>VNVLGGIEYSINNATLCSVGFSVTRGATKGFVTAGHCGGVGAIVRIGGTQVGSFAARVFPGNDRAWVSVGSAHTLQGAVSNYSGGTIAIRGSAEAAIGAAVCRSGRTTGYRCGNITAKNVTANYAEGAVRGLTQGNACMGRGDSGGSWFTSAGQAQGVMSGGNVQSNGNNCGIPASQRSSLFERVGPILSQYGLSLVTS[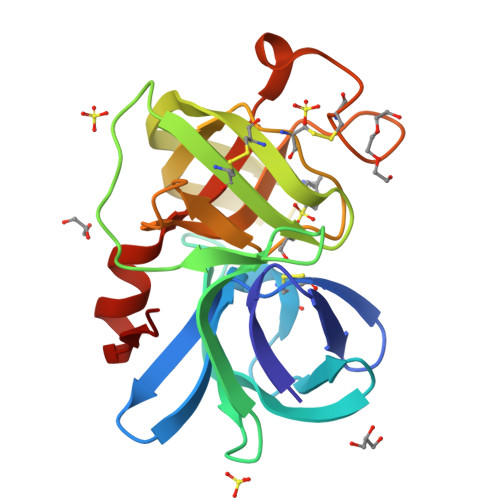4x]>[2x]AECSVDIQGNDQMQYNTNAITVDKSCKQFTVNLSHPGNLPKNVMGHNFVLSTAADMQGVVTDGMASGLDKDFLKPDDSRVIAQTKLIGSGEKDSVTFD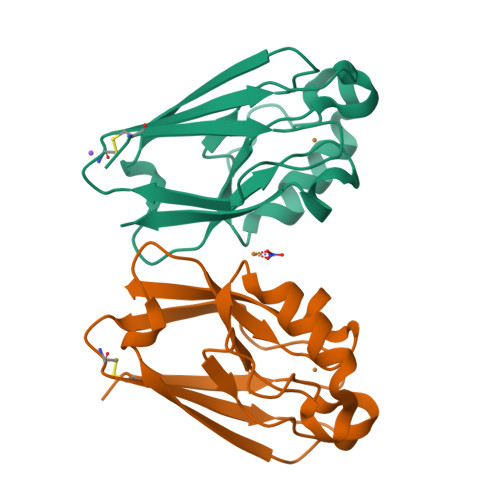VSKLKEGEQFMFFCTFPGHSALMKGHLTLK[(2R,3S,5R)-3-hydroxy-5-(5-methyl-2,4-dioxo-3,4-dihydropyrimidin-1(2H)-yl)tetrahydrofuran-2-yl]methyl 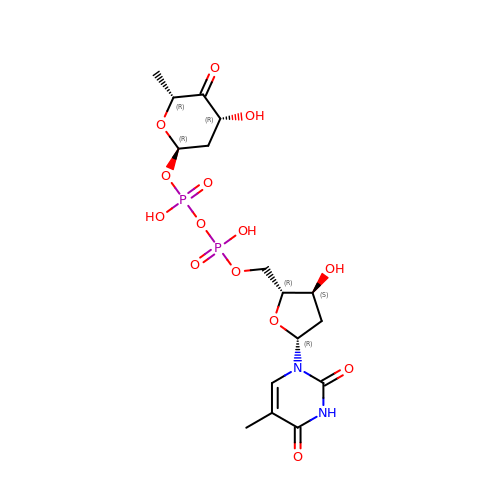(2R,4R,6R)-4-hydroxy-6-methyl-5-oxotetrahydro-2H-pyran-2-yl dihydrogen diphosphate | C16 H24 N2 O14 P2 | AONILRCSLAIOQE-LREJFELKSA-N Two groups of enzymes, muramidases and N-acetylglucosaminidases, cleave alternate but chemically equivalent glycosidic bonds in the NAG-NAM polymers. The S. aureus Mu50 genome (an MRSA strain with vancomycin-intermediate resistance; VISA) encodes five N-acetyl­glucosaminidases belonging to glycoside hydrolase family 73 (GH73 family). The crystal structure of AtlE and its complexes with substrate fragments described here provide insight into the mechanism of NAG-NAM binding, whereas a comparison with structural data for lysozymes and their complexes with substrate fragments enabled us to seek out the structural differences responsible for docking of the two alternate glycosidic bonds in the NAG-NAM polymer. The compact α-helical structural core forms the lower part of both domains, whereas the R-lobe and L-lobe contain short α-helical and β-strand regions, respectively.

The structure has additional five amino acids (SNAAA) at the N-terminus remaining after cleavage of the His tag by TEV protease. In the MDP complex the NAM and alanine residues are unambiguously resolved by the electron-density map, whereas the positioning of the atoms of the d-glutamic acid residue is less defined, as indicated by the electron-density map. The O atom of the lactyl moiety of the NAM residue forms a hydrogen bond to the OH group of the Tyr201 side chain. The alanine hydrophobic side chain is positioned within the hydrophobic environment formed by the side chains of Ile163, Gly164 and Phe196, whereas the d-glutamic acid residue is disordered and points into the solvent. The superimposed structures show similar positioning of the carbohydrate rings, yet different positions and orientations of the peptidyl extensions (the T4 muropeptide in green is pointing to the right and the AtlE-bound muropeptide MDP in red is pointing to the left), which provide insight into the difference in specificity between N-acetylgluco­s­aminidases and muramidases. The opposite positioning of the lactyl moieties in the active sites of the N-acetylglucosaminidase AtlE and the muramid­ase ACOD predicts that features on the left side of the active-site cleft of AtlE are responsible for the recognition of lactyl moieties and peptides from the glycopeptides, whereas the features on the right side of the active-site cleft of AtlE should prevent the binding of lactyl moieties and peptides attached to them. The reverse is true for ACOD substrate binding. Indeed, Figs. 8(a) and 8(b) show that in the L-lobe and above the −2 and +1 positions of the lactyl moieties of NAM residues bound to the AtlE surface, there is sufficient space to accommodate the peptidyl extensions. The absence of AtlE activity against NAG substrates can be attributed to the extended but not twisted conformation of the NAG substrate, which disables productive binding at the −3 and −2 positions.

> SAAANDVNYSFDEAVSMQQGKGIVQTKEEDGKFVEANNNEIAKAMTISHKDNDMKYMDITEKVPMSESEVNQLLKGKGILENRGKVFLEAQEKYEVNVIYLVSHALVETGNGKSELAKGIKDGKKRYYNFFGIGAFDSSAVRSGKSYAEKEQWTSPDKAIIGGAKFIRNEYFENNQLNLYQMRWNPENPAQHQYASDIRWADKIAKLMDKSYKQFGIKKDDIRQTYYK>GSMEKSMSPFVKKHFVLVHTAFHGAWCWYKIVALMRSSGHNVTALDLGASGINPKQALQIPNFSD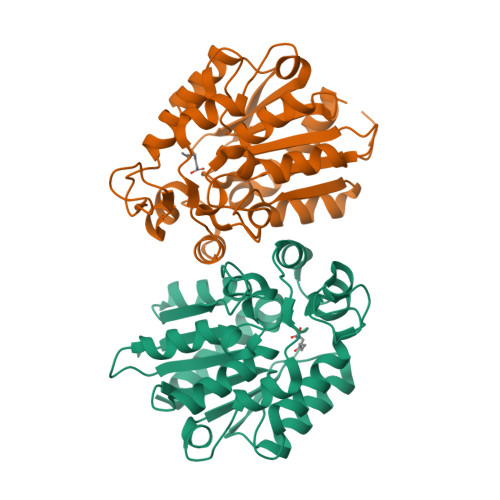YLSPLMEFMASLPANEKIILVGHALGGLAISKAMETFPEKISVAVFLSGLMPGPNIDATTVCTKAGSAVLGQLDNCVTYENGPTNPPTTLIAGPKFLATNVYHLSPIEDLALATALVRPLYLYLAEDISKEVVLSSKRYGSVKRVFIVATENDALKKEFLKLMIEKNPPDEVKEIEGSDAVTMMSKPQQLFTTLLSIANKYK[2x]>[3x]MDAELKIFVSSQHQPDIWRKALDQYEAKTPGVKVVIETGGNTSEMQAQYLNTVMSAKDSSLDVLMLDVIRPAQFATAGWTSDFSGKDLSAYLPTYAEANTVNGKIVALPAFADSMFLYYRKDLLDKYGIKPPTTWDELKEASKKVMEGEKNPELQGLSFQGKAIEGAVCTFLLPYWSEGKSLVENGKLNFDNKAAVDSLKLWKSFVDDGISKKNISEVATDDTRKEF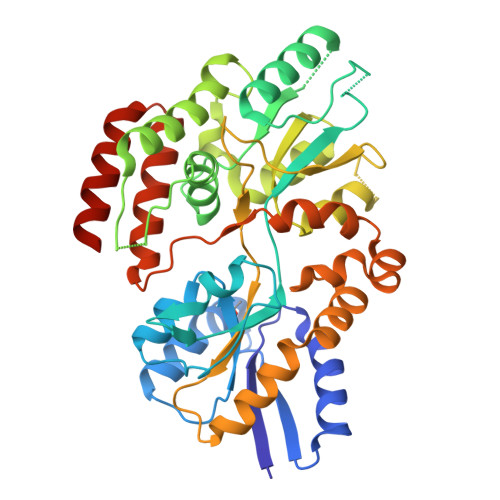QAGKVLFAVNWSYAWTHFQGKESQVNDKVGVARLPAVKGGEQTTCLGGWEFGVSAYSKQQDEAKKLVEYLSSQDVSKFMAINAALLPTYAALYKDADVTKTIPWFADALPVVETAKARPVTPRYNEVSETIRTTVNGVLAGVMTPEDGAKQMESRLRRVLRLEHHHHHH4-(2-azaspiro[3.4]octan-2-ylmethyl)-~{N}-[[(3~{R})-3-oxidanyl-1-[6-[(phenylmethyl)amino]pyrimidin-4-yl]piperidin-3-yl]methyl]benzamide | C32 H40 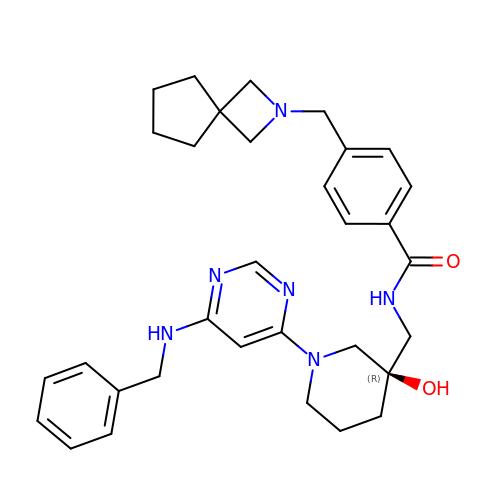N6 O2 | SVCYBAWPGFFEQO-JGCGQSQUSA-N>MKIFFITSNPGKVRE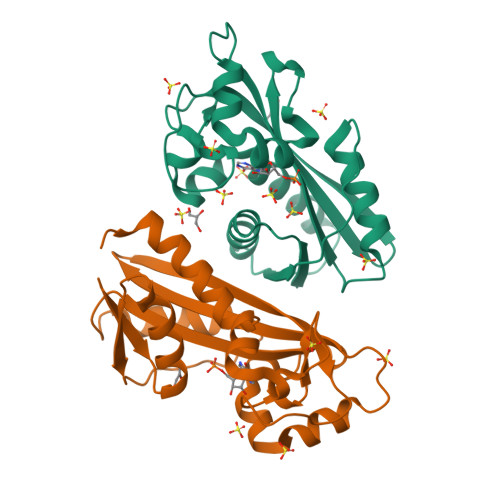VANFLGTFGIEIVQLKHEYPEIQAEKLEDVVDFGISWLKGKVPEPFMIEDSGLFIESLKGFPGVYSSYVYRTIGLEGILKLMEGAEDRRAYFKSVIGFYIDGKAYKFSGVTWGRISNEKRGTHGFGYDPIFIPEGSEKTFAEMTIEEKNALSHRGKALKAFFEWLKVNLKY[2x]>[2x]MAISLATKAATDALKVNRAPVGVEPQEVHKWLQSFNWDFKENRTKYATKYHMANQTKEQFKVIAKEYARMEAAKDERQFGTLLDGLTRLGAGNKVHPRWGETMKVISNFLEVGEYNAIAASAMLWDSATAAEQKNGYLAQVLDEIRHTHQCAFINHYYSKHYHDPAGHNDARRTRAIGPLWKGMKRVFADGFISGDAVECSVNLQLVGEACFTNPLIVAVTEWASANGDEITPTVFLSVETDELRHMANGYQTVVSIANDPAAAKYLNTDLNNAFWTQQKYFTPALGYLFEYGSKFKVEPWVKTWNRWVYEDWGGIWIGRLGKYGVESPRSLRDAKTDAYWAHHDLALAAYALWPLGFAR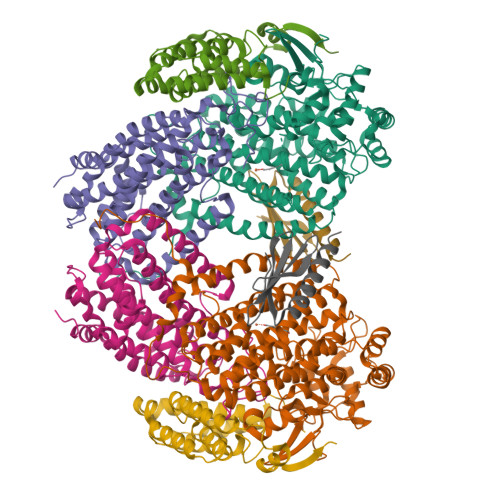LALPDEEDQEWFEANYPGWADHYGKIYNEWKKLGYEDPKSGFIPYAWLLANGHDVYIDRVSQVPFIPSLAKGSGSLRVHEFNGKKHSLTDDWGERMWLSEPERYECHNLFEQYEGRELSEVIAEGHGVRSDGKTLIAQPHVRGDNLWTLEDIKRAGCVFPNPLAKF;>[2x]MSQPQSSQVTKRGLTDPERAAIIAAAVPDHALDTQRKYHYFIQPRWKRLSEYEQLSCYAQPNPDWIAGGLDWGDWTQKFHGGRPSWGNESTELRTTDWYRHRDPARRWHAPYVKDKSEEARYTQRFLAAYSSEGSIRTIDAYWRDEILNKYYGALLYNEYGLFNAHSSVGRDCLSDTIRQSATFAGLDKVDNAQMIQMERLFIAKLVPGFDASTDVPKKIWTTDPIYAGARGAVEEIWQGIQDWNEILWAGHAVYDATFGQFARREFFQRLATVYGDTLTPFFTAQSQTYFQTTRGAIEDLFVYCLANDPEFGAHNRTFLNAWTEHYLARSVTALKDFVGIYAKVEKVAGATDRAGVSEALQRVFGDWKVDYADKIGFNIDVDQKVDAVLAGFKN;>MAKREPIHENSTRTEWEGKIAKLNSVDQATKFIQDFRVAYSSPFRKSYDLDVDYQYIERKIEERLSVLKTEKLSVADLVTKATTGEDAAAVEAAWIAKMKAAESKYAAERIHIEFRQLYKPPVLPVNVFLRTDAALGTILMELRNTDYYATPLEGLRKERGVKVLHLQA[2x];>[2x]SNAMAHSAEPTTEASRILIHSDARYEAFTVDLDYMWRWEILRDGEFVQEGCSLSFDSSRKAVAHVLSHFKRQDEAAQRPGDNSAEIKRLLQSLGTPIPVNEQNDSTKNELAQPE> SDEVRKNLMDMFRDRQAFSEHTWKMLLSVCRSWAAWCKLNNRKWFPAEPEDVR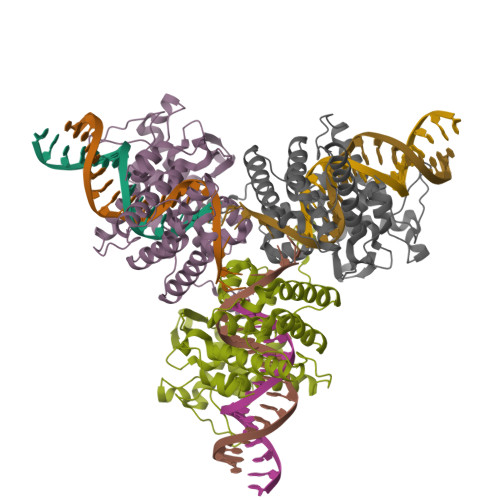DYLLYLQARGLAVKTIQQHLGQLNMLHRRSGLPRPSDSNAVSLVMRRIRKENVDAGERAKQALAFERTDFDQVRSLMENSDRCQDIRNLAFLGIAYNTLLRIAEIARIRVKDISRTDGGRMLIHIGRTKTLVSTAGVEKALSLGVTKLVERWISVSGVADDPNNYLFCRVRKNGVAAPSATSQLSTRALEGIFEATHRLIYGAKDDSGQRYLAWSGHSARVGAARDMARAGVSIPEIMQAGGWTNVNIVMNFIRNLDSETGAMVRLLEDGD To gain insights into the molecular mechanisms that govern the metalloreductase activity of STEAP proteins, we determine structures of human STEAP4 using single-particle cryo-EM. The trimeric structures reveal an aligned, inter-subunit NADPH-FAD-heme arrangement and suggest that chelated iron(III) binds in a cavity of basic residues to facilitate reduction. Our biochemical and structural characterization of human STEAP4 elucidated that detergent-solubilized STEAP4 forms trimers that exhibit ferric-reductase activity in the presence of its redox cofactors, FAD and heme, and electron donor, NADPH, indicating that the enzyme does not require specific accessory proteins for catalysis. The trimeric arrangement observed in the cryo-EM structures is formed by interactions in STEAP protomers in both the OxRD and TMD layers, with a phospholipid molecule packed in between the TMDs of adjacent enzyme subunits, indicating that lipids stabilize the trimer.

We then determined structures of STEAP4EM in the presence of NADPH and FAD (cofactor-bound state) and in the presence of NADP+, FAD, and Fe3+-NTA (cofactor/substrate-bound state) using single-particle cryo-EM. The cofactor and cofactor/substrate-bound datasets yielded reconstructed density maps at 3.8 and 3.1 Å resolution, respectively. Binding of substrate Fe3+-NTA does not induce conformational rearrangements in STEAP4, because the densities of the cofactor/substrate and the cofactor-bound structures are virtually identical. Nevertheless, a prominent and highly significant density, positioned directly above the porphyrin in each protomer, is observed in a difference map between the two reconstructions. STEAP4 residues are positioned far beyond ~2.0-Å from the center of the difference density, indicating no direct interactions of Fe3+ with residues of enzyme. Instead, we observed nine basic amino acids surrounding the difference density at 4.5–9 Å distances. These residues form a positively charged, ~16-Å wide ring that is consistent with binding of Fe3+, while it remains in complex with a negatively charged chelator like NTA or citrate. We propose that this ring-shaped arrangement of basic amino-acid residues provides a second coordination shell, which may facilitate metal reduction by controlling the position of chelated Fe3+ with respect to the heme, and by modulating the polarity of the iron-chelator complex, thereby making Fe3+ more susceptible to electron uptake. Although the current data does not allow to accurately model the substrate in the density, it is obvious that binding of iron(III), by itself, in this electropositive environment is highly unfavorable. This implies that STEAPs reduce iron while it remains in complex with a negatively charged chelator.

>MEKTCIDALPLTMNSSEKQETVCIFGTGDFGRSLGLKMLQCGYSVVFGSRNPQKTTLLPSGAEVLSYSEAAKKSGIIIIAIHREHYDFLTELTEVLNGKILVDISNNLKINQYPESNAEYLAHLVPGAHVVKAFNTISAWALQSGALDASRQVFVCGNDSKAKQRVMDIVRNLGLTPMDQGSLMAAKEIEKYPLQLFPMWRFPFYLSAVLCVFLFFYCVIRDVIYPYVYEKKDNTFRMAISIPNRIFPITALTLLALVYLPGVIAAILQLYRGTKYRRFPDWLDHWMLCRKQLGLVALGFAFLHVLYTLVIPIRYYVRWRLGNLTVTQAILKKENPFSTSSAWLSDSYVALGILGFFLFVLLGITSLPSVSNAVNWREFRFVQSKLGYLTLILCTAHTLVYGGKRFLSPSNLRWYLPAAYVLGLIIPCTVLVIKFVLIMPCVDNTLTRIRQGWERNSKH[3x]1-beta-D-ribofuranosyl-1,3,5-triazinane-2,4,6-trione | C8 H11 N3 O7 | 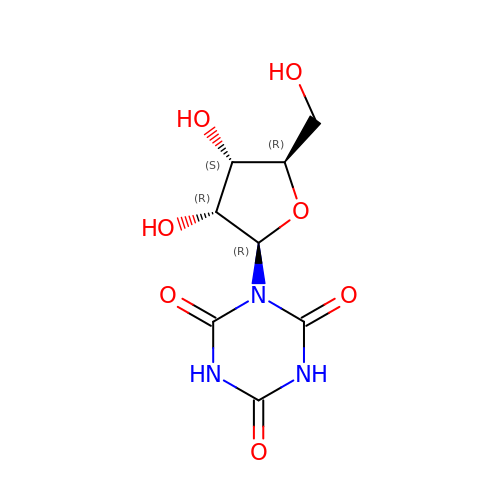DKOBRNXETUUICC-TXICZTDVSA-N> MLIRRLKDARLRAGISQEKLGVLAGIDEASASARMNQYEKGKHAP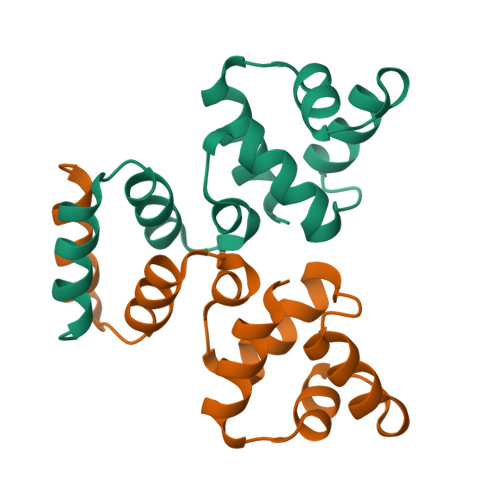DFEMANRLAKVLKIPVSYLYTPEDDLAQIILTWNELNEQERKRINFYIRKKAK> GIDPFTKHGQKECDNALRQLETVRELLENPVQPINDMSYFGCLDSVMENSKVLGEAMTGISQNAKNGNLPEFGDAIATASKALCGFTEAAAQAAYLVGVSDPNSQAGQQGLVEPTQFARANQAIQMACQSLGEPGCTQAQVLSAATIVAKHTSALCNSCRLASARTANPTAKRQFVQSAKEVANSTANLVKTIKALDGDFTEENRAQCRAATAPLLEAVDNLSAFASNPEFSSVPAQISPEGRAAMEPIVISAKTMLESAGGLIQTARALAVNPRDPPRWSVLA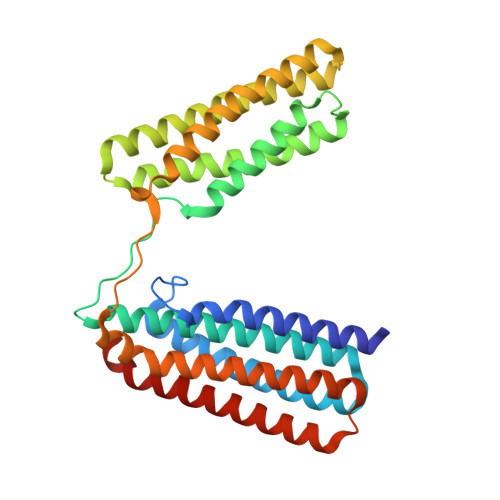GHSRTVSDSIKKLITSMRDKAPGQL> SMKLDIKKTFSNRSDRVKGIDFHPTEPWVLTTLASGRVEIWNYETQVEVRSIQVTETPVRAGK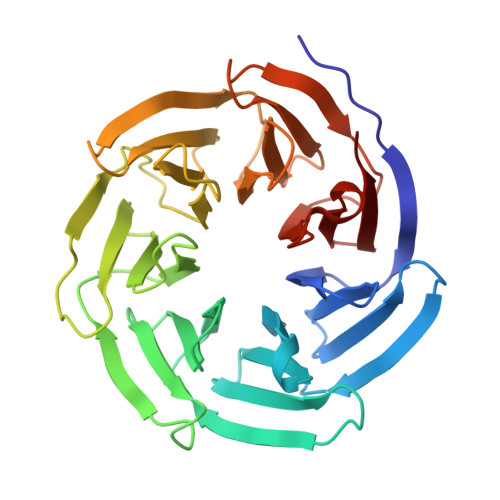FIARKNWIIVGSDDFRIRVFNYNTGEKVVDFEAHPDYIRSIAVHPTKPYVLSGSDDLTVKLWNWENNWALEQTFEGHEHFVMCVAFNPKDPSTFASGCLDRTVKVWSLGQSTPNFTLTTGQERGVNYVDYYPLPDKPYMITASDDLTIKIWDYQTKSCVATLEGHMSNVSFAVFHPTLPIIISGSEDGTLKIWNSSTYKVEKTLNVGLERSWCIATHPTGRKNYIASGFDNGFTVLSLG>[4x]MGRLVGLELSNFKSYRGVTKVGFGESNFTSIIGPNGSGKSNMMDAISFVLGVRSNHLRSNILKDLIYRGVLNDENSDDYDNEGAASSNPQSAYVKAFYQKGNKLVELMRIISRNGDTSYKIDGKTVSYKDYSIFLENENILIKAKNFLVFQGDVEQIAAQSPVELSRMFEEVSGSIQYKKEYEELKEKIEKLSKSATESIKNRRRIHGELKT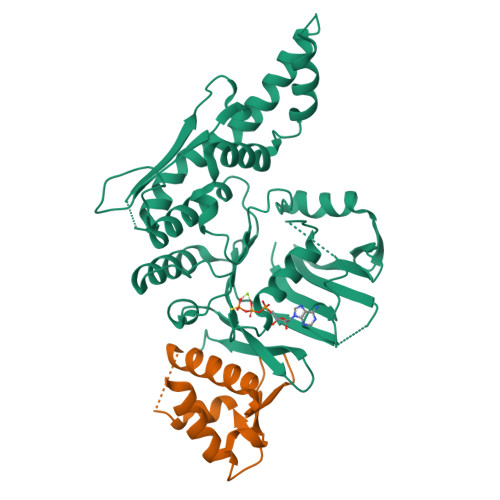YKSPGLEVLFQGPRGSRYDEAEGRFEVINNETEQLKAEEKKILNQFLKIKKKRKELFEKTFDYVSDHLDAIYRELTKNPNSNVELAGGNASLTIEDEDEPFNAGIKYHATPPLKRFKDMEYLSGGEKTVAALALLFAINSYQPSPFFVLDEVDAALDITNVQRIAAYIRRHRNPDLQFIVISLKNTMFEKSDALVGVYRQQQENSSKIITLDLSNYAE;>[4x]MHHHHHHFPEENIIDAKTRNEQTTIQTEKVRPTPGEVASKAIVQMAKILRKELSEEKEVIFTDVLKSQANTEPENITKREASRGFFDILSLATEGCIGLSQTEAFGNIKIDAKPALFERFI>[4x]SMKQDSRFPNLFILDHPLIQHKLTHMRDKDTSTRTFRELLREITLLMGYEITRNLPITTKRVETPLVEIDAP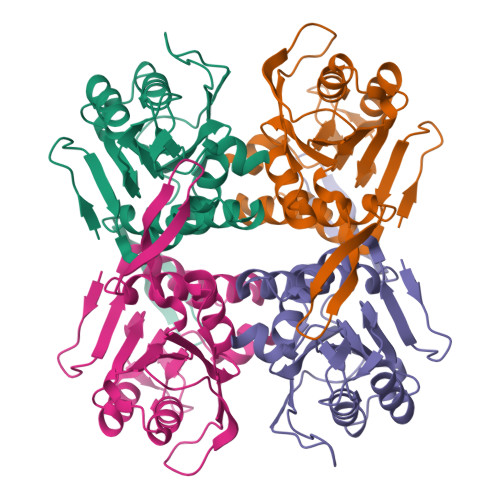VIAGKKLAIVPVLRAGVGMSDGLLELIPSARVGHIGVYRADDHRPVEYLVRLPDLEDRIFILCDPMVATGYSAAHAIDVLKRRGVPGERLMFLALVAAPEGVQVFQDAHPDVKLYVASLDSHLDDHAYIVPGLGDAGDRLFGTKN>GMLPKLVITHRVHEEILQLLAPHCELITNQTDSTLTREEILRRCRDAQAMMAFMPDRVDADFLQACPELRVIGCALKGFDNFDVDACTARGVWLTFVPDLLTVPTAELAIGLAVGLGRHLRAADAFVRSGQFRGWQPRFYGTGLDNATVGFLGMGAIGLAMADRLQGWGATLQY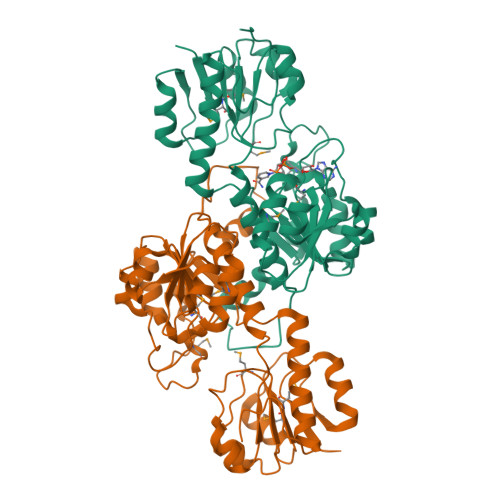HAAKALDTQTEQRLGLRQVACSELFASSDFILLALPLNADTLHLVNAELLALVRPGALLVNPCRGSVVDEAAVLAALERGQLGGYAADVFEMEDWARADRPQQIDPALLAHPNTLFTPHIGSAVRAVRLEIERCAAQNILQALAGERPINAVNRLPKANP[6x]> SNAMGQQSGAVYVGNYRVVNRHLAT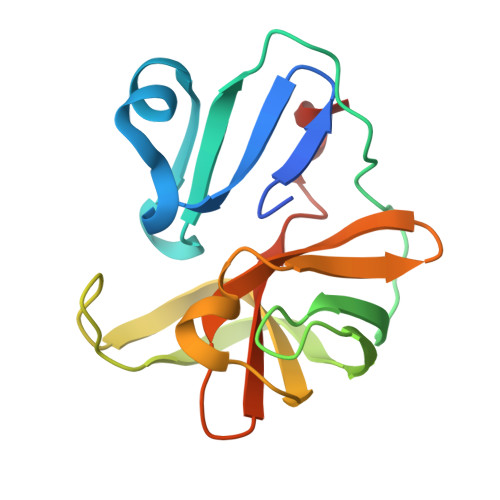SADWQNCVWESYNRDLLVSTTTAHGCDIIARCQCTTGVYFCASKNKHYPISFEGPGLVEVQESEYYPRRYQSHVLLAAGFSEPGDAGGILRCEHGVIGIVTMGGEGVVGFADIRDLLWLEDDAMEQ>[8x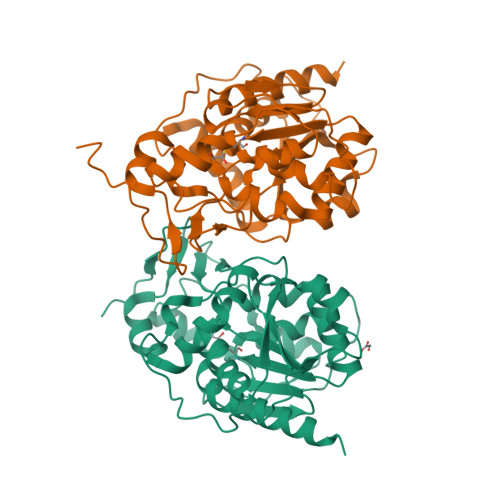]MSQDVNELSKQPTPDKAEDNAFFPSPYSLSQYTAPKTDFDGVEHKGAYKDGKWKVLMIAAEERYVLLENGKMFSTGNHPVEMLLPLHHLMEAGFDVDVATLSGYPVKLELWAMPTEDEAVISTYNKLKEKLKQPKKLADVIKNELGPDSDYLSVFIPGGHAAVVGISESEDVQQTLDWALDNDRFIVTLXHGPAALLSAGLNREKSPLEGYSVCVFPDSLDEGANIEIGYLPGRLKWLVADLLTKQGLKVVNDDMTGRTLKDRKLLTGDSPLASNELGKLAVNEMLNAIQNKLEHHHHHH Herein, a type of exolytic heparinases (exoHepases) is identified from the genomes of different bacteria. These exoHepases share almost no homology with known Hepases and prefer to digest HP rather than HS chains by sequentially releasing unsaturated disaccharides from their reducing ends. The structure of BIexoHep consists of three domains: an N-terminal small β-sheet domain (Ala24–Asn150) composed of a large loop and a five-stranded β-sheet (β1–β5), a central (α/α)5 barrel domain (Pro151–Glu515) containing 20 α-helices (α1–α20) to form an (α/α)5 incomplete toroid structure, and a C-terminal β-sandwich domain (Leu516–Pro864) containing 23 β-strands and 5 short α-helices that fold into a three-layered β-sheet sandwich structure (α21–α25 and β6–β28). Further structural studies have shown that the active center of the exolytic Hepase is an L-shaped semiopen tunnel with a positively charged entrance and a negatively charged exit, which precisely controls the sequential cleavage of highly negatively charged HP.

Furthermore, a crystal of an inactive BIexoHep-Y390A/H555A mutant with an unsaturated HP tetrasaccharide substrate was obtained, and the structure was solved at a resolution of 1.73 Å by molecular replacement with Phaser using the complex structure of BIexoHep with the product as a template. In the crystal structures, each asymmetric unit consists of one BIexoHep monomer, an unsaturated disaccharide (ΔUA2S1-4GlcNS6S) or tetrasaccharide (ΔUA1-4GlcNS6S1-4IdoA2S1-4GlcNS6S), and two Ca2+ ions that were confirmed by inductively coupled plasma-mass spectrometry (ICP-MS) analysis. Notably, the BIexoHep complex with the disaccharide product and the structure with the tetrasaccharide substrate do not show significant differences (the root-mean-square deviation (r.m.s.d.) between the two structures was 0.140 Å based on 786 atoms). According to the hydrogen-bonding networks, a series of residues, such as Asp70, Ser226, Arg230, Arg233, Arg332, Asn336, His337, Gln340, Tyr390, Ser554, His555, Arg579, Arg648, Lys755, and Arg757, participate in the binding of the disaccharide product (ΔUA2S1-4GlcNS6S) and the tetrasaccharide substrate (ΔUA1-4GlcNS6S1-4IdoA2S1-4GlcNS6S). The reducing end sugar rings of the tetrasaccharide substrate at the +1 and +2 subsites are tightly hugged by the side chains of the residues in the positively charged section of the L-shaped tunnel via a hydrogen bond network. In contrast, the nonreducing end sugar rings at subsites −1 and −2 have fewer direct interactions with the residue sidechains because the “+” subsites are deeply buried in the tunnel, while the “−” subsites are exposed to the environment. The residues His337, Tyr390 and His555 match well with three key residues His202, Tyr257 and His406 in the active center of Hepase II from P. heprinus DSM 2366, indicating that they may also play key roles in the catalytic mechanism of BIexoHep.

> MKKIILGLSVLCLLMACGSSEQPAVIKVSEETLMYEVRATPSPADGTYVKVNPPRFMWPDKFPHLGPVLDGVPGQVDEKPKVVYRIRISQDKNFRKDVLTGERAWAFFNPFQCLAQGKWYWQHAYVTPEGTEEWSPVYQFYIDKDTPEFNPPTLEKVLARYPSHHPRVLLDADDWENIIAKNNNNPEARTYMDKASQCISRPLKHLQEEIDTTNVVTLTNIVQRESALIRESRKIVDREEANVEALVRAYLLTKDEKYYREGINRLSEILSWQKSKYFAGDFNLSTLLSMSTSAYDGFYNLLSPEEKQLLLDNIRKIGDKFYNEYVNHLENRIADNHVWQMTFRILTMAAFATVGEIPEASVWTDYCYNEWISRLPGLHKDGGWHNGDAAFHVNIRTLIEVPVFFSRISGFNFFADPWYNNNALYVIYQQPPFSKSGGHGNSHEGQRSPNGGRIGYADALARECNNPWAAAYVHEIMQEDPDILSKAFEAKPADLTWYRCTTPKERPAYSKHLSELPESKVFKQTGTALMNTDIGHHANNAMLSFRSSPYGSTSAALANQNAFNTFFGGKAIFYSSGHRTGFTDDHCMYAYRNTRAHNSILVNGMGQKIGTEGYGWIPRYYEGEEISYVVGDASNAYGKVVSPLWLERGRLSGTQFTPEKGWDENKLEFFRRHVVQLGRSGLFVVYDELAGKEPVEWNYLLHTVELPMEVVKEEGGLRILGKNKADGISIAHLYSSQEMTYAQTDTFFVAALDWKKRLGKALPNHYHFTATTAPCNKVFFLNIIDVHGNNRADAVINHQGNHITVEGWVIECNLDSEGKAFLHIENKQNGASLDFNYNSNKGATTIVDQVDGKRIEKRLVDSLPEPEILEHHHHHH> MSQDRILLDLDVVNQRLILFNSAFPSDAIEAPFHFSNKESTSENLDNLAGTILHSRSITGHVFLYKHIFLEIVARWIKDSKKKDYVLVIEKLASIITIFPVAMPLIEDYLDKENDHFITILQNPSTQKDSDMFKILLAYYRLLYHNKEVFARFIQPDILYQLVDLLTKEQENQVVIFLALKVLSLYLDMGEKTLNDMLDTYIKSRDSLLGHFEGDSGIDYSFLELNEAKRCANFSKLPSVPECFTIEKKSSYFIIEPQDLSTKVASICGVIVPKVHTIHDKVFYPLTFVPTHKTVSSLRQLGRKIQNSTPIMLIGKAGSGKTFLINELSKYMGCHDSIVKIHLGEQTDAKLLIGTYTSGDKPGTFEWRAGVLATAVKEGRWVLIEDIDKAPTDVLSILLSLLEKRELTIPSRGETVKAANGFQLISTVRINEDHQKDSSNKIYNLNMIGMRIWNVIELEEPSEEDLTHILAQKFPILTNLIPKLIDSYKNVKSIYMNTKFISLNKGAHTRVVSVRDLIKLCERLDILFKNNGINKPDQLIQSSVYDSIFSEAADCFAGAIGEFKALEPIIQAIGESLDIASSRISLFLTQHVPTLENLDDSIKIGRAVLLKEKLNIQKKSMNSTLFAFTNHSLRLMEQISVCIQMTEPVLLVGETGTGKTTVVQQLAKMLAKKLTVINVSQQTETGDLLGGYKPVNSKTVAVPIQENFETLFNATFSLKKNEKFHKMLHRCFNKNQWKNVVKLWNEAYKMAQSILKITNTENENENAKKKKRRLNTHEKKLLLDKWADFNDSVKKFEAQSSSIENSFVFNFVEGSLVKTIRAGEWLLLDEVNLATADTLESISDLLTEPDSRSILLSEKGDAEPIKAHPDFRIFACMNPATDVGKRDLPMGIRSRFTEIYVHSPERDITDLLSIIDKYIGKYSVSDEWVGNDIAELYLEAKKLSDNNTIVDGSNQKPHFSIRTLTRTLLYVTDIIHIYGLRRSLYDGFCMSFLTLLDQKSEAILKPVIEKFTLGRLKNVKSIMSQTPPSPGPDYVQFKHYWMKKGPNTIQEQAHYIITPFVEKNMMNLVRATSGKRFPVLIQGPTSSGKTSMIKYLADITGHKFVRINNHEHTDLQEYLGTYVTDDTGKLSFKEGVLVEALRKGYWIVLDELNLAPTDVLEALNRLLDDNRELFIPETQEVVHPHPDFLLFATQNPPGIYGGRKILSRAFRNRFLELHFDDIPQDELEIILRERCQIAPSYAKKIVEVYRQLSIERSASRLFEQKNSFATLRDLFRWALRDAVGYEQLAASGYMLLAERCRTPQEKVTVKKTLEKVMKVKLDMDQYYASLEDKSLEAIGSVTWTKGMRRLSVLVSSCLKNKEPVLLVGETGCGKTTICQLLAQFMGRELITLNAHQNTETGDILGAQRPVRNRSEIQYKLIKSLKTALNIANDQDVDLKELLQLYSKSDNKNIAEDVQLEIQKLRDSLNVLFEWSDGPLIQAMRTGNFFLLDEISLADDSVLERLNSVLEPERSLLLAEQGSSDSLVTASENFQFFATMNPGGDYGKKELSPALRNRFTEIWVPSMEDFNDVNMIVSSRLLEDLKDLANPIVKFSEWFGKKLGGGNATSGVISLRDILAWVEFINKVFPKIQNKSTALIQGASMVFIDALGTNNTAYLAENENDLKSLRTECIIQLLKLCGDDLELQQIETNEIIVTQDELQVGMFKIPRFPDAQSSSFNLTAPTTASNLVRVVRAMQVHKPILLEGSPGVGKTSLITALANITGNKLTRINLSEQTDLVDLFGADAPGERSGEFLWHDAPFLRAMKKGEWVLLDEMNLASQSVLEGLNACLDHRGEAYIPELDISFSCHPNFLVFAAQNPQYQGGGRKGLPKSFVNRFSVVFIDMLTSDDLLLIAKHLYPSIEPDIIAKMIKLMSTLEDQVCKRKLWGNSGSPWEFNLRDTLRWLKLLNQYSICEDVDVFDFVDIIVKQRFRTISDKNKAQLLIEDIFGKFSTKENFFKLTEDYVQINNEVALRNPHYRYPITQNLFPLECNVAVYESVLKAINNNWPLVLVGPSNSGKTETIRFLASILGPRVDVFSMNSDIDSMDILGGYEQVDLTRQISYITEELTNIVREIISMNMKLSPNATAIMEGLNLLKYLLNNIVTPEKFQDFRNRFNRFFSHLEGHPLLKTMSMNIEKMTEIITKEASVKFEWFDGMLVKAVEKGHWLILDNANLCSPSVLDRLNSLLEIDGSLLINECSQEDGQPRVLKPHPNFRLFLTMDPKYGELSRAMRNRGVEIYIDELHSRSTAFDRLTLGFELGENIDFVSIDDGIKKIKLNEPDMSIPLKHYVPSYLSRPCIFAQVHDILLLSDEEPIEESLAAVIPISHLGEVGKWANNVLNCTEYSEKKIAERLYVFITFLTDMGVLEKINNLYKPANLKFQKALGLHDKQLTEETVSLTLNEYVLPTVSKYSDKIKSPESLYLLSSLRLLLNSLNALKLINEKSTHGKIDELTYIELSAAAFNGRHLKNIPRIPIFCILYNILTVMSENLKTESLFCGSNQYQYYWDLLVIVIAALETAVTKDEARLRVYKELIDSWIASVKSKSDIEITPFLNINLEFTDVLQLSRGHSITLLWDIFRKNYPTTSNSWLAFEKLINLSEKFDKVRLLQFSESYNSIKDLMDVFRLLNDDVLNNKLSEFNLLLSKLEDGINELELISNKFLNKRKHYFADEFDNLIRYTFSVDTAELIKELAPASSLATQKLTKLITNKYNYPPIFDVLWTEKNAKLTSFTSTIFSSQFLEDVVRKSNNLKSFSGNQIKQSISDAELLLSSTIKCSPNLLKSQM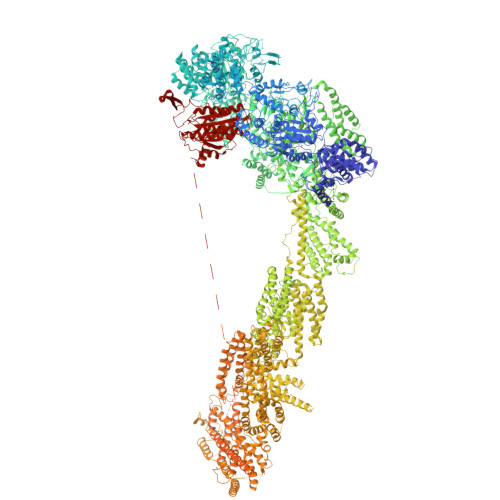EYYKNMLLSWLRKVIDIHVGGDCLKLTLKELCSLIEEKTASETRVTFAEYIFPALDLAESSKSLEELGEAWITFGTGLLLLFVPDSPYDPAIHDYVLYDLFLKTKTFSQNLMKSWRNVRKVISGDEEIFTEKLINTISDDDAPQSPRVYRTGMSIDSLFDEWMAFLSSTMSSRQIKELVSSYKCNSDQSDRRLEMLQQNSAHFLNRLESGYSKFADLNDILAGYIYSINFGFDLLKLQKSKDRASFQISPLWSMDPINISCAENVLSAYHELSRFFKKGDMEDTSIEKVLMYFLTLFKFHKRDTNLLEIFEAALYTLYSRWSVRRFRQEQEENEKSNMFKFNDNSDDYEADFRKLFPDYEDTALVTNEKDISSPENLDDIYFKLADTYISVFDKDHDANFSSELKSGAIITTILSEDLKNTRIEELKSGSLSAVINTLDAETQSFKNTEVFGNIDFYHDFSIPEFQKAGDIIETVLKSVLKLLKQWPEHATLKELYRVSQEFLNYPIKTPLARQLQKIEQIYTYLAEWEKYASSEVSLNNTVKLITDLIVSWRKLELRTWKGLFNSEDAKTRKSIGKWWFYLYESIVISNFVSEKKETAPNATLLVSSLNLFFSKSTLGEFNARLDLVKAFYKHIQLIGLRSSKIAGLLHNTIKFYYQFKPLIDERITNGKKSLEKEIDDIILLASWKDVNVDALKQSSRKSHNNLYKIVRKYRDLLNGDAKTIIEAGLLYSNENKLKLPTLKQHFYEDPNLEASKNLVKEISTWSMRAAPLRNIDTVASNMDSYLEKISSQEFPNFADLASDFYAEAERLRKETPNVYTKENKKRLAYLKTQKSKLLGDALKELRRIGLKVNFREDIQKVQSSTTTILANIAPFNNEYLNSSDAFFFKILDLLPKLRSAASNPSDDIPVAAIERGMALAQSLMFSLITVRHPLSEFTNDYCKINGMMLDLEHFTCLKGDIVHSSLKANVDNVRLFEKWLPSLLDYAAQTLSVISKYSATSEQQKILLDAKSTLSSFFVHFNSSRIFDSSFIESYSRFELFINELLKKLENAKETGNAFVFDIIIEWIKANKGGPIKKEQKRGPSVEDVEQAFRRTFTSIILSFQKVIGDGIESISETDDNWLSASFKKVMVNVKLLRSSVVSKNIETALSLLKDFDFTTTESIYVKSVISFTLPVITRYYNAMTVVLERSRIYYTNTSRGMYILSTILHSLAKNGFCSPQPPSEEVDDKNLQEGTGLGDGEGAQNNNKDVEQDEDLTEDAQNENKEQQDKDERDDENEDDAVEMEGDMAGELEDLSNGEENDDEDTDSEEEELDEEIDDLNEDDPNAIDDKMWDDKASDNSKEKDTDQNLDGKNQEEDVQAAENDEQQRDNKEGGDEDPNAPEDGDEEIENDENAEEENDVGEQEDEVKDEEGEDLEANVPEIETLDLPEDMNLDSEHEESDEDVDMSDGMPDDLNKEEVGNEDEEVKQESGIESDNENDEPGPEEDAGETETALDEEEGAEEDVDMTNDEGKEDEENGPEEQAMSDEEELKQDAAMEENKEKGGEQNTEGLDGVEEKADTEDIDQEAAVQQDSGSKGAGADATDTQEQDDVGGSGTTQNTYEEDQEDVTKNNEESREEATAALKQLGDSMKEYHRRRQDIKEAQTNGEEDENLEKNNERPDEFEHVEGANTETDTQALGSATQDQLQTIDEDMAIDDDREEQEVDQKELVEDADDEKMDIDEEEMLSDIDAHDANNDVDSKKSGFIGKRKSEEDFENELSNEHFSADQEDDSEIQSLIENIEDNPPDASASLTPERSLEESRELWHKSEISTADLVSRLGEQLRLILEPTLATKLKGDYKTGKRLNMKRIIPYIASQFRKDKIWLRRTKPSKRQYQIMIALDDSKSMSESKCVKLAFDSLCLVSKTLTQLEAGGLSIVKFGENIKEVHSFDQQFSNESGARAFQWFGFQETKTDVKKLVAESTKIFERARAMVHNDQWQLEIVISDGICEDHETIQKLVRRARENKIMLVFVIIDGITSNESILDMSQVNYIPDQYGNPQLKITKYLDTFPFEFYVVVHDISELPEMLSLILRQYFTDLASS> MKNDYRTFKLSLLTLAPIHIGNGEKYTSREFIYENKKFYFPDMGKFYNKMVEKRLAEKFEAFLIQTRPNARNNRLISFLNDNRIAERSFGGYSISETGLESDKNPNSAGAINEVNKFIRDAFGNPYIPGSSLKGAIRTILMNTTPKWNNENAVNDFGRFPKENKNLIPWGPKKGKEYDDLFNAIRVSDSKPFDNKSLILVQKWDYSAK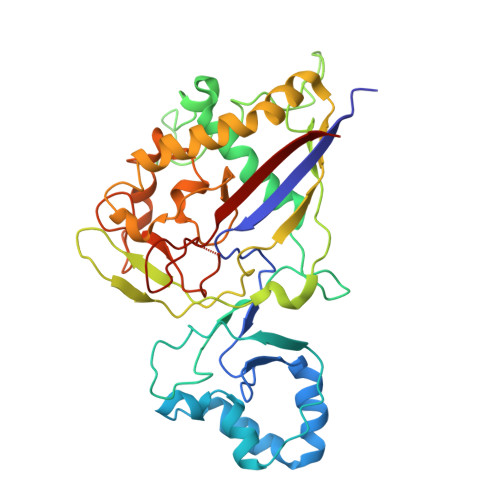TNKAKPLPLYRESISPLTKIEFEITTTTDEAGRLIEELGKRAQAFYKDYKAFFLSEFPDDKIQANLQYPIYLGAGSGAWTKTLFKQADGILQRRYSRMKTKMVKKGVLKLTKAPLKTVKIPSGNHSLVKNHESFYEMGKANFMIKEIDK> MELKHSISD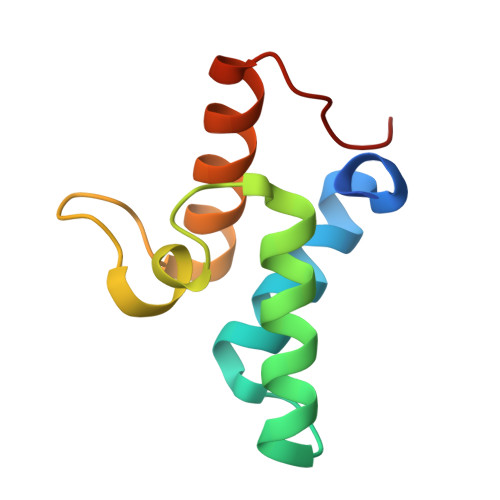YTEAEFLQLVTTICNADTSSEEELVKLVTHFEEMTEHPSGSDLIYYPKEGDDDSPSGIVNTVKQWRAANGKSGFKQG> MVDQATLDKLEAGFKKLQEASDCKSLLKKHLTKDVFDSIKNKKTGMGATLLDVIQSGVENLDSGVGIYAPDAESYRTFGPLFDPIIDDYHGGFKLTDKHPPKQWGDINTLVDLDPAGQFIISTRVRCGRSLQGYPFNPCLTA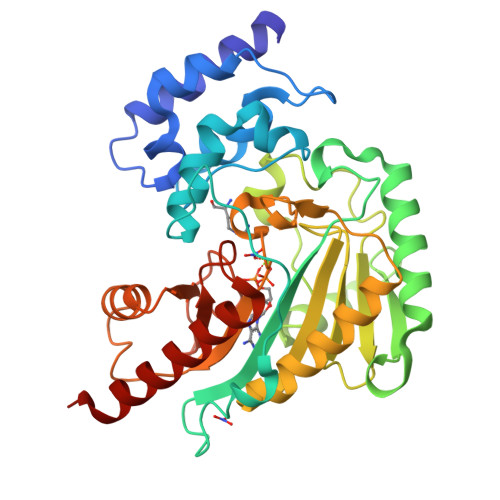EQYKEMEEKVSSTLSSMEDELKGTYYPLTGMSKATQQQLIDDHFLFKEGDRFLQTANACRYWPTGRGIFHNDAKTFLVWVNEEDHLRIISMQKGGDLKTVYKRLVTAVDNIESKLPFSHDDRFGFLTFCPTNLGTTMRASVHIQLPKLAKDRKVLEDIASKFNLQVRGTRGDHTESEGGVYDISNKRRLGLTEYQAVREMQDGILEMIKMEKAAA> IIGGREVIPHSRPYMASLQRNGSHLCGGVLVHPKWVLTAAHCLAQRMAQLRLVLGLHTLDSPGLTFHIKAAIQHPRYKPVPALENNLALLQLDGKVKPSRTIRPLALPSKRQVVAAGTRCSMAGWGLTHQGGRLSRVLRELDLQVLDTRMCNNSRFWNGSLSPSMVCLAADSKDQAPCKGDSGGPLVCGKGRVLAGVLSFSSRVCTDIFKPPVATAVAPYVSWIRKVTGRSALEHHH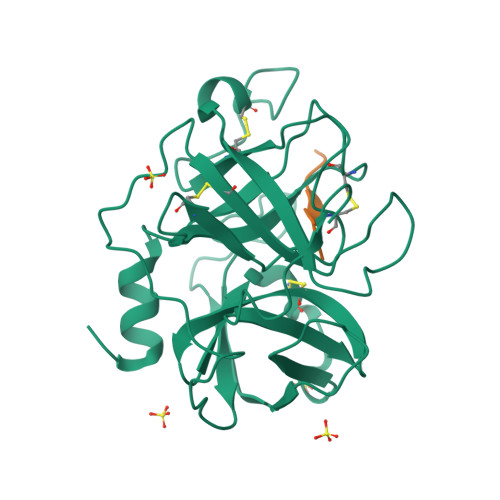HHH;> SSGKVPLS>ITQTLELSDLTIALEEFERYGITERMIIVLKNIQKIVAKNKLCNLNELKFSSLSRELKLFEELLKIPSPPEKIANSIYKINDILESSIREFKLCSKNSENLFFIKPIQKFLVDFQKIVLEKLPLDKKINKYSNIATLEKVEFMKNIIKLLINWKMYSEAVIHLRELLIDIKLIENGKYFYYNNKDFREKYWMYSYNIVDTKDKELPKKIEELLKNVKGWRNSVAHGGRANTSINQKTLEENLENALSMIDEILLSMKDLKVNSKKIYLLNSTIMPIPKDNQEGKFYILKLTKNEFKVILENAIKDDVLDSAIGHESVIEFIKDKFELTVPLKRKEI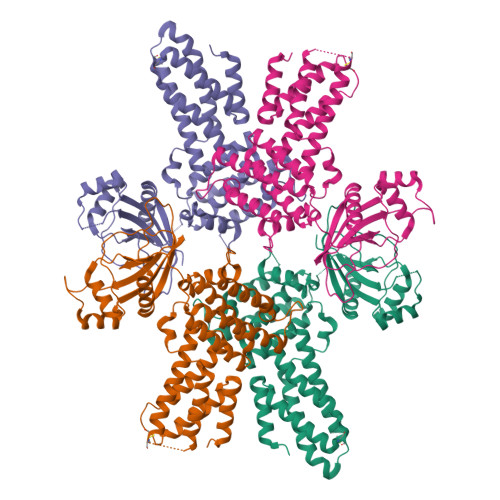YFEKGESALVIKLEKRPEEGKIYTKEEMDFMEENNLIGYYYIYREG[2x]> MAPSRANTSVIVVGGGGTIGSSTALHLVRSGYTPSNVTVLDAYPIPSSQSAGNDLAKIMGVSLRNPVDLQLALEARQMWNEDELFKKFFHNTGRLDCAHGEKDIADLKSGYQALVDAGLDATNEWLDSEDEILKRMPLLSRDQIKGWKAIFSKDGGWLAAAKAINAVGEYLRDQGVRFGFYGAGSFKAPLLAEGVCIGVETVDGTRYYADKVVLAAGAWSPTLVELHEQCVSKAWVYGHIQLTPEEAARYKNSPVVYNGDVGFFFEPNEHGVIKVCDEFPGFTRFKMHQPFGAKAPKRISVPRSHAKHPTDTIPDASDVSIRRAIATFMPQFKNKKMFNQAMCWCTDTADAALLICEHPEWKNFVLATGDSGHSFKLLPNIGKHVVELLEGTLADDLAHAWRWRPGSGDALKSRRSAPAKDLADMPGWNHDKPRANLLEHHHHHH

N-valyl-histidine derived from proteolytic digestion of the N-terminus of the HbA1c β-chain. This study reports the X-ray structures of the wild-type and Asn56Ala (N56A) mutant of Phaeosphaeria nodorum fructosyl peptide oxidase (PnFPOX) to elucidate the residues responsible for the oxidative half-reaction. Fructosyl amine oxidases (FAOXs) are FAD-containing enzymes that catalyze the oxidative deglycosylation of fructosyl amino acids such as fructosyl valine and/or ε-fructosyl lysine, which are the degradation products of HbA1c and GA, respectively. As members of the FAOX family, fructosyl peptide oxidases (FPOXs) are also known as candidates for diagnostic enzymes. A covalent bond is formed between FAD and Cys343 of PnFPOX as observed in amadoriase I (Cys342), amadoriase II (Cys335), and EtFPOX (Cys347).

N56A showed decreased oxidase activity compared to the wild -type, while its dye-mediated dehydrogenase activity was higher than that of wild type. In PnFPOX N56A, Lys274, and Asp54 approach each other, and the water molecule is displaced from the W2 position such that Lys274 forms salt bridges with Asp54 at 2.92–3.35 Å. The relocated Asp54 also forms water (W3′ and W4′)-mediated hydrogen bond with His239 and is stabilized in this position. However, with the movement of Asp54 and Lys274 in PnFPOX N56A, the corresponding space no longer provides enough room to bind with a water molecule (W2). The analysis of the protein channels of the structures showed that the W1, W2, and W4 positions in wild-type PnFPOX (W1′ and W4′ in PnFPOX N56A) are in the main oxygen-accessible channel. In PnFPOX N56A, the movement of Asp54 and Lys274 blocks a short and plausible main channel observed in wild-type PnFPOX (blue dotted path with arrow in Supplementary Figure S6). Although the oxygen could be accessible through another alternative long path instead of the closed path in PnFPOX N56A, the elimination of the accessibility toward the short pathway might result the drastic decrease in oxidase activity compared with dye-mediated dehydrogenase activity. Comparison of active site structures between wild-type PnFPOX with bound acetate and PnFPOX N56A revealed no significant differences. The observed increase in dye-mediated dehydrogenase activity in PnFPOX N56A can be explained by the decrease in competition between the dye mediator and oxygen. Our structural comparison revealed that Asn56 in PnFPOX has a crucial role in assisting and stabilizing the oxygen path involving Asp54, Lys57, and Lys274 in terms of oxidase activity. This comparison also suggests that Asn56 in PnFPOX is essential for properly maintaining a plausible main oxygen channel and oxidase activity involved in the movement of Lys274.>GSHMTPEHLPTEQYEAQLAEKVVRLQSMMAPFSDLVPEVFRSPVSHYRMRAEFRIWHDGDDLYHIIFDQQTKSRIRVDSFPAASELINQLMTAMIAGVRNNPVLRHKLFQIDYLTTLSNQAVVSLLYHKKLDDEWRQEAEALRDALRAQNLNVHLIGRATKTKIELDQDYIDERLPVAGKEMIYRQVENSFTQPNAAMNIQMLEWALDVTKGSKGDLLELYCGNGNFSLALARNFDRVLATEIAKPSVAAAQYNIAANHIDNVQIIRMAAEEFTQAMNGVREFNRLQGIDLKSYQCETIFVDPPRSGLDSETEKMVQAYPRILYISCNPETLCKNLETLSQTHKVERLALFD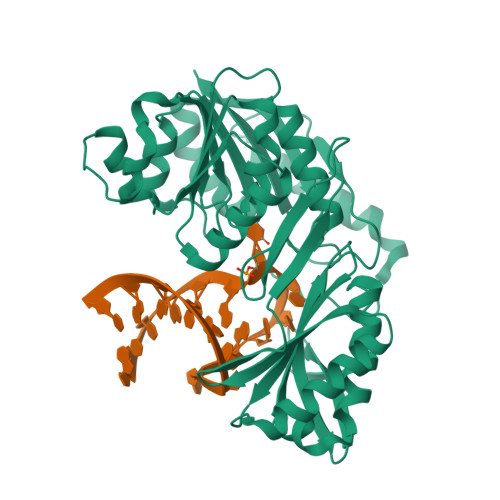QFPYTHHMQCGVLLTAK[2x]> MMQPSIKPADEHSAGDIIARIGSLTRMLRDSLRELGLDQAIAEAAEAIPDARDRLYYVVQMTAQAAERALNSVEASQPHQDQMEKSAKALTQRWDDWFADPIDLADARELVTDTRQFLADVPAHTSFTNAQLLKIMMAQDFQDLTGQVIKRMMDVIQEIERQLLMVLLENIPEQESRPKRENQSLLNGPQVDTSKAG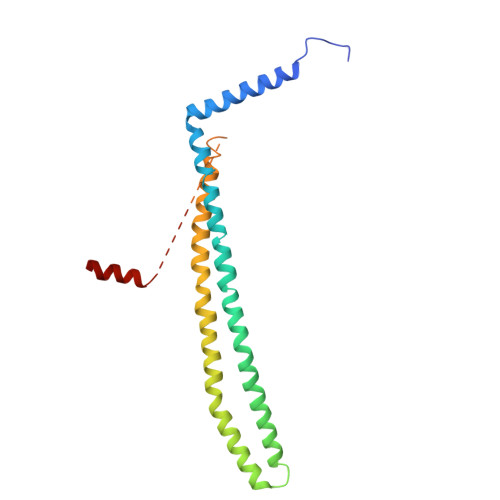VVASQDQVDDLLDSLGF> SDEFDALRIKWATLLTGGPALDPADSDIAARTDKLAQDANDYWEDMDLSSSRTYIWYALRGNGTSDNVNAVYERLRTMALAATTVGSSLYGNADLKEDILDALDWLYVNSYNSTRSRSAYNWWHWQLGIPMSLNDIAVLLYDDISAARMATYMDTIDYFTPSIGLTGANRAWQAIVVGVRAVIVKDAVKLAAARNGLSGTGIFPYATGGDGFYADGSFVQHTTFAYTGGYGSSVLETTANLMYLLSGSTWSVSDPNQSNVWQWIYEAYRPLLYKGAMMDMVRGREISRSYAQDHAVGHGIVASIVRLAQFAPAPHAAAFKQIAKRVIQEDTFSSFYGDVSTDTIRLAKAIVDDPSIAPAAAPNLYKQYAAMDRAVLQRPGFALGLALYSTRISSYESINSENGRGWYTGAGATYLYNQDLAQYSEDYWPTVDAYRIPGTTVASGTPIASGTGTSSWTGGVSLAGQYGASGMDLSYGAYNLSARKSWFMFDDEIVALGSGISS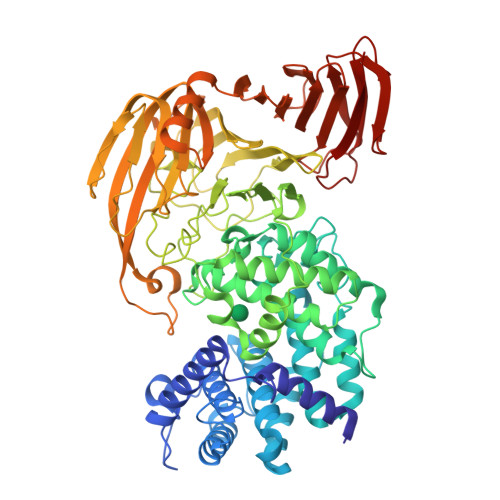TAGIPIETVVDNRKLNGAGDNAWTANGAALSTGLGVAQTLTGVNWVHLAGNTADGSDIGYYFPGGATLQTKREARTGTWKQINNRPATPSTAVTRNYETMWIDHGTNPSGASYGYVLLPNKTSAQVGAYAADPAIEIVVNTSGVQSVKEKTLGLVGANFWTDTTQTADLITSNKKASVMTREIADERLEASVSDPTQANNGTIAIELARSAEGYSADPGITVTQLAPTIKFTVNVNGAKGKSFHASFQLG5-(dodecylthio)-1H-1,2,3-triazole-4-carboxylic 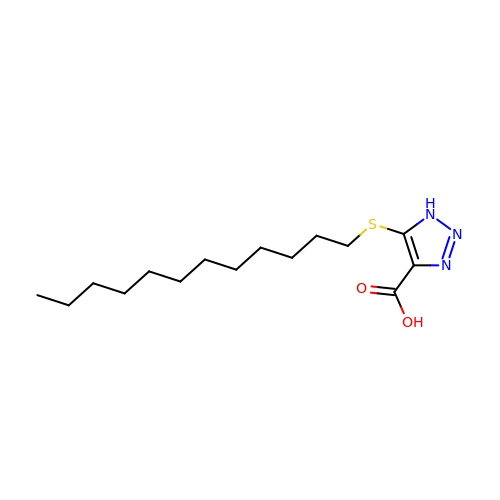acid | C15 H27 N3 O2 S | IEZPFPQAXAREGM-UHFFFAOYSA-N>MFDPKKFIDEAVEEIKQQISDRKAIIALSGGVDSSVAAVLTHKAIGDKLTAVFVDTGLMRKGEREEVEKTFRDKLGLNLIVVDAKDRFLNALKGVTDPEEKRKIIGKLFIDVFEEIAEDIKAEVLVQGTIAPDWIETQGKIKSHHNVALPHGMVLEVVEPLRELYKDEVRLLAKELGLPDSIVYRQPFPGPGLAVRVLGEVTEEKLNICREANAIVEEEVKKANLDKDLWQYFAVVLDCKATGVKGDEREYNWIVALRMVKSLDAMTAHVPEI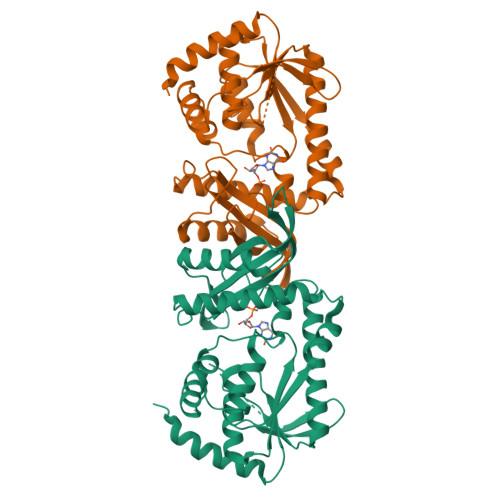PFDLLKRISKRITSEIPNVARVVFDITDKPPATIEFE[4x]> MSHLDKVQPVIKNSDMSVEMQKEVEEVAKKAIDYCNTDKEIATFIKDDFRSRYHGTWHCIVGRNFGSFVTFERSYY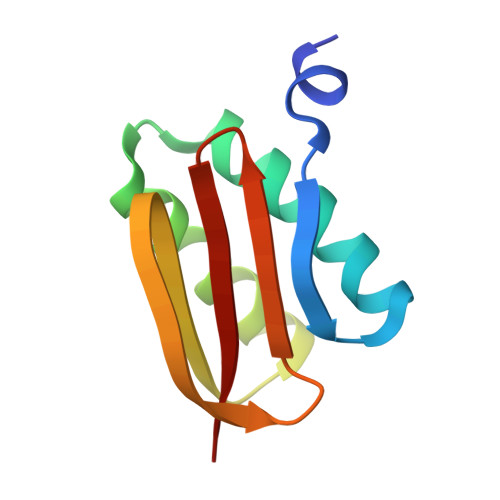IYLYVGQLAILLFKTG>GHMSTLLINQPQYAWLKELGLREENEGVYNGSWGGRGEVITTYCPANNEPIARVRQASVADYEETVKKAREAWKIWADIPAPKRGEIVRQIGDALREKIQVLGSLVSLEMGKILVEGVGEVQEYVDICDYAVGLSRMIGGPILPSERSGHALIEQWNPVGLVGIITAFNFPVAVYGWNNAIAMICGNVCLWKGAPTTSLISVAVTKIIAKVLEDNKLPGAICSLTCGGADIGTAMAKDERVNLLSFTGSTQVGKQVGLMVQERFGRSLLELGGNNAIIAFEDADLSLVVPSALFAAVGTAGQRCTTARRLFIHESIHDEVVNRLKKAYAQIRVGNPWDPNVLYGPLHTKQAVSMFLGAVEEAKKEGGTVVYGGKVMDRPGNYVEPTIVTGLGHDASIAHTETFAPILYVFKFKNEEEVFAWNNEVKQGLSSSIFTKDLGRIFCWLGPKGSDCGIVNVNIPTSGAEI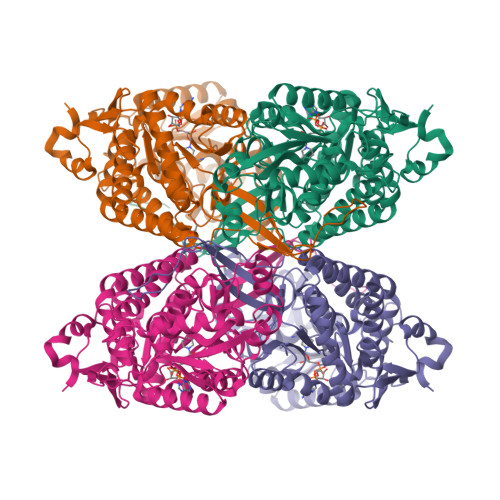GGAFGGEKHTGGGRESGSDAWKQYMRRSTCTINYSKDLPLAQGIKFQ[8x]(2~{S})-~{N}-[(1~{S})-1-[4-[(6-pyridin-4-ylquinazolin-2-yl)amino]phenyl]ethyl]piperidine-2-carboxamide 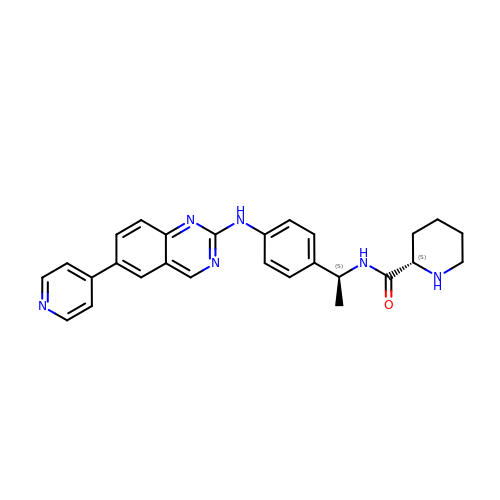| C27 H28 N6 O | OQQHJQAFUOXHSI-BVZFJXPGSA-N>[3x]SSPADSYNEGVKLQPQEISPPPTANLDRSNDKVYENVTGLVKAVIEMSSKIQP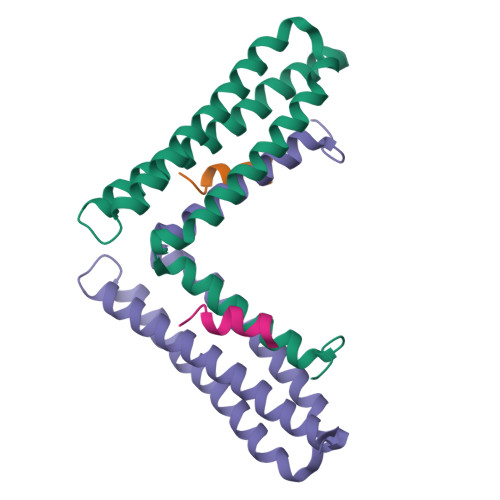APPEEYVPMVKEVGLALRTLLATVDETIPLLPASTHREIEMAQKLLNSDLGELINKMKLAQQYVMTSLQQEYKKQMLTAAHALAVDAKNLLDVIDQARLKMLGQTRPH;>[2x]ATRELDELMASLS>X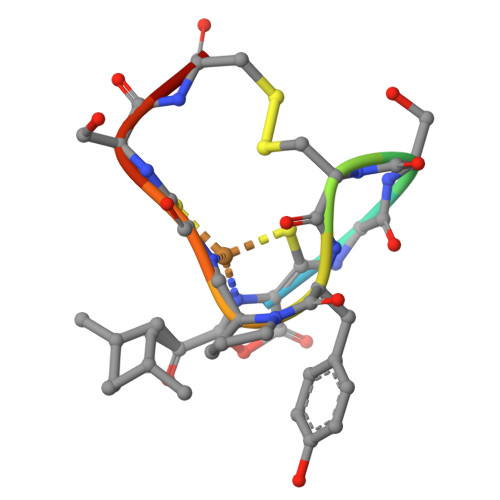CGSCYPCSCM[6x]>SNAMLRRLFKKKYVCVRQYDLTDCGAACLSSIAQYYGLKMSLAKIREMTGTDTQGTNAYGLIHAAKQLGFSAKGVKASKEDLLKDFRLPAIANVIVDNRLAHFVVIYSIKNRIITVADPGKGIVRYSMDDFCSIWTGGLVLLEPGEAFQKGDYTQNMMVKFAGFLKPLKKTVLCIFLASLLYTALGIAGSFYIKFLFDDLIKFEKLNDLHIISAGFAVIFLLQIFLNYYRSILVTKLGMSIDKSIMMEYYSHVLKLPMNFFNSRKVGEIISRFMDASKIRQAISGATLTIMIDTIMAVIGGILLYIQNSSLFFISFIIILLYGIIVTVFNKPIQNANRQIMEDNAKLTSALVESVKGIETIKSFGAEEQTEKSTRDKIETVMKSSFKEGMLYINLSSLTGIVAGLGGIVILWAGAYNVIKGNMSGGQLLAFNALLAYFLTPVKNLIDLQPLIQTAVVASNRLGEILELATEKELREDSDDFVISLKGDIEFRNVDFRYGLRKPVLKNINLTIPKGKTVAIVGESGSGKTTLAKLLMNFYSPEKGDILINGHSIKNISLELIRKKIAFVSQDVFIFSGTVKENLCLGNENVDMDEIIKAAKMANAHDFIEKLPLKYDTFLNESGANLSEGQKQRLAIARALLKKPDILILDEATSNLDSITENHIKDAIYGLEDDVTVIIIAHRLSTIVNCDKIYLLKDGEIVESGSHTELIALKGCYFKMWKQTENTLAS[2x];>[2x]SNAMSEAKKLNIGRELTDEELMEMTGGSTFSIQCQKDYTYKPSLPVVKYGVVIDEPEVVIKYGVGPIVGIKYGVEPIGPIQPMYGIKPVETLK

Peptidase-containing ABC transporters (PCATs) in gram-positive bacteria function both as maturation proteases and exporters for biofilm formation, quorum sensing, or antimicrobial polypeptides. Substrates of PCATs are synthesized as precursors with an N-terminal leader peptide. Proteolytic cleavage of the leader peptide at the conserved double-glycine motif is necessary for secretion of the cargo peptide. In this work, we determined the structures of wild-type PCAT1 (wtPCAT1) in the presence of substrate and ATP with or without Mg2+.

To analyze the conformational states of PCAT1 under ATP turnover conditions, cryo-EM samples were prepared using wtPCAT1 mixed with twofold molar excess of the substrate CtA, 10 mM ATP-Mg2+, and the creatine phosphate ATP-regenerating system. Among the 671,000 particles analyzed by three-dimensional (3D) classification, ∼83% exhibit IF conformations with different degrees of NBD separation, 14% are in an NBD-dimerized configuration, and the remaining 3% do not show any protein features. Subsequent refinement resulted in a low-resolution (6.6-Å) NBD-dimerized structure and three molecular structures of NBD-separated IF conformations, referred to as IF wide (IFW, 4.1 Å), intermediate (IFI, 3.7 Å), and narrow (IFN, 3.7 Å), respectively. The three IF structures share a similar overall conformation, in which the two PEP domains dock symmetrically onto the intracellular openings of the TM cavity. The leader peptide (residues 8 to 24) of the substrate forms an L-shaped structure wrapping around the PEP domain. The double-glycine cleavage site (G23/G24) is positioned on a narrow cleft on PEP in close proximity to the catalytic triad residues C21, H99, and D115. Consistently, the density inside the TM cavity is separated from both leader peptides, indicating that the cargo peptide inside the TM cavity has been freed from its leader peptide. Densities consistent with ATP and Mg2+ were observed in all three reconstructions. Different from the NBD-dimerized structure, in the NBD-separated conformations, ATP binds to the Walker A/B motifs of one NBD, distant from the ABC signature motif of the opposite NBD. The majority of PCAT1 adopts an IF conformation in which the NBDs are separated, the substrate is enclosed inside the TM cavity, and the PEP domains remain associated with the transporter core.>[4x]LHMVPALTREQLYIFDTTGFLVIPGVFGSGEVESFRSELERLDTVDPGFPRTRRYPDLPAASPVFARL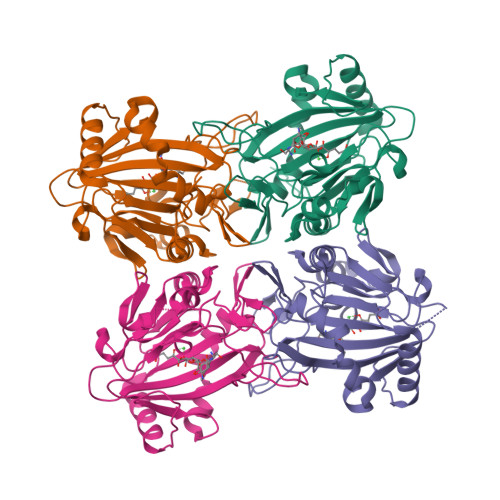ALDDRLLAPVRDVVNQPLRLLEGYGLRRTKDSVLYLHGGNSELLDLGDRQVGRDLSITHTYHDGKLYCPYVKALVYLSDIQSPEDGSFCYVQGSHKANFPLLRERAERGENTSLVDSGFPTLSDVFVRSGDVLLLNEALMHGTRRKLTEGDRLLTAFGYGPTFFTEWRELDAETADLRGAGYVDHDVEEDFVL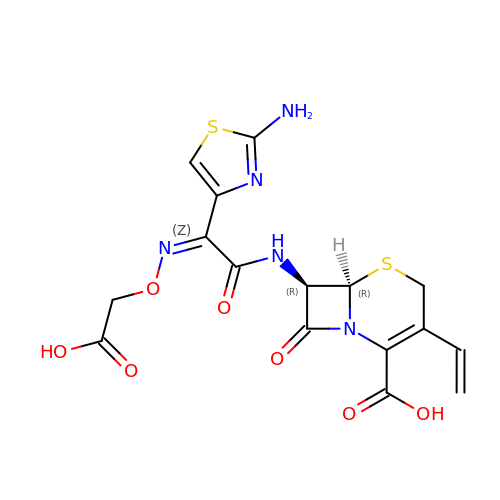(6R,7R)-7-({(2Z)-2-(2-amino-1,3-thiazol-4-yl)-2-[(carboxymethoxy)imino]acetyl}amino)-3-ethenyl-8-oxo-5-thia-1-azabicyclo[4.2.0]oct-2-ene-2-carboxylic acid | C16 H15 N5 O7 S2 | OKBVVJOGVLARMR-QSWIMTSFSA-N The human AIP gene encodes a 37 kDa protein of 330 amino acids that, based on similarities to other proteins, is predicted to have an N-terminal immunophilin-like domain and a C-terminal tetratricopeptide repeat (TPR) domain. The TPR domain of AIP is similar to other TPR-domain proteins consisting of three pairs of anti-parallel helices and a Cα-7h. We present the structure showing the molecular interactions of the TPR domain of AIP in complex with the peptide-binding motifs of HSP90 and TOMM20. We found that the EDASRMEEVD (HSP90) and AQSLAEDDVE (TOMM20) peptides bind within the TPR-domain cleft and adopt a similar backbone conformation.

Interactions between the TOMM20 peptide and the TPR domain of AIP are similar but not identical. The main differences result due to the need to pack the first glutamate side-chain of the TOMM20 peptide (AQSLAEDDVE) into the hydrophobic pocket that accepts the methionine residue in the case of HSP90 peptide (MEEVD). While the side chain of this glutamate enters the hydrophobic pocket the carboxylate oxygens point back towards and interacts with the side-chain amine of Lys 266. Consequently, Lys 266 adopts an alternative conformation to that seen with the HSP90 bound peptide. The conformational change in Lys 266 acts like a switch that not only allows the binding of the TOMM20 glutamate in the methionine pocket, but also allows the longer C-terminal glutamate side-chain of TOMM20 (Asp in HSP90), to pack between the side chain of Pro 232 and Lys 266; and consequently form a hydrogen bond via a water molecule with the side-chain amine of Asn 264. Significantly, Arg 304, whose missense mutation is linked to disease, was found to form interactions with the aspartates of the TOMM20 peptide (AQSLAEDDVE) bound in the neighbouring TPR domain. The structure with TOMM20 peptide showed that electron density for residues Asp 172 to Arg 325 of the TPR domain was visible. Structural analysis showed that the Gln 307 and Arg 325 amino acid residues (all clearly visible in the TOMM20-AIP structure), are further away from the TPR domain-binding site than Arg 304, and are not involved in packing interactions or in binding of the bound conserved peptide motifs. Thus, the rearrangement that allows the glutamate residue of TOMM20 (EDDVE) to bind the hydrophobic pocket also allows the longer C-terminal glutamate side-chain of TOMM20 to be accommodated. * 10-mer peptides were used in the crystallization, but only 6–7 resides were visible.

>[2x]DPWAMTAEEKAKAVPLIHQEGNRLYREGHVKEAAAKYYDAIACLKNLQMKEQPGSPEWIQLDQQITPLLLNYCQCKLVVEEYYEVLDHCSSILNKYDDNVKAYFKRGKAHAAVWNAQEAQADFAKVLELDPALAPVVSRELQALEARIRQKDEEDKARFRGIFSH;>AEDDVE[2x]> MAQILPIRFQEHLQLQNLGINPANIGFSTLTMESDKFICIREKVGEQAQVVIIDMNDPSNPIRRPISADSAIMNPASKVIALKAGKTLQIFNIEMKSKMKAHTMTDDVTFWKWISLNTVALVTDNAVYHWSMEGESQPVKMFDRHSSLA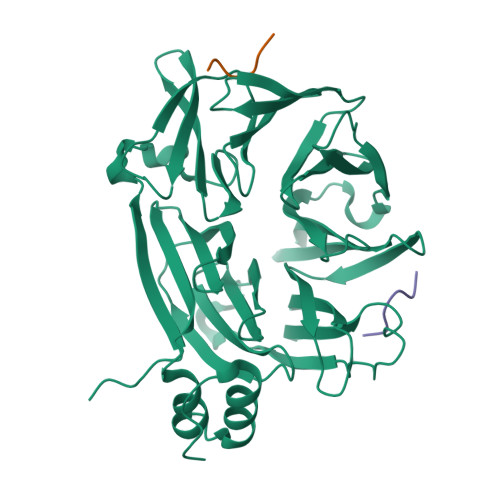GCQIINYRTDAKQKWLLLTGISAQQNRVVGAMQLYSVDRKVSQPIEGHAASFAQFKMEGNAEESTLFCFAVRGQAGGKLHIIEVGTPPTGNQPFPKKAVDVFFPPEAQNDFPVAMQISEKHDVVFLITKYGYIHLYDLETGTCIYMNRISGETIFVTAPHEATAGIIGVNRKGQVLSVCVEEENIIPYITNVLQNPDLALRMAVRNNLAGAEEL;>[2x]DQLIDL>GPGSEFMGAWLRAIGLERYEEGLVHNGWDDLEFLSDITEEDLEEAGVQDPAHKRLLLDTLQLSKSSGENLYFQSSGSSGGSSGSEGVPFRTVSEWLESIKMQQYTEHFMVAGYTAIEKVVQMSNEDIKRIGVRLPGHQKRIAYSLLGLKDQVNTVGIPI[2x]

The Eph (erythropoietin-producing hepatocyte) transmembrane receptor tyrosine kinase superfamily, with its first member identified30 years ago, contains 14 members in mammals and is the largest among all receptor tyrosine kinase families. However, the cytoplasmic portion of all 14 Eph receptors are highly similar, each containing a membrane-juxtaposing kinase domain, a protein-binding SAM domain immediately followed by a short carboxyl tail PDZ domain-binding motif (PBM). In this study, we performed systematic biochemical and structural studies of the bindings of three SAM domains, two from previously identified Eph-binding proteins (SHIP2 and Odin) and one from a new Eph-binding protein discovered in this study (SAMD5), to the SAM domains from every Eph receptor. Our study reveals that the Eph SAM domains have exquisitely specific target SAM domain-binding properties, although their overall SAM-SAM heterodimer formation modes are very similar.

ITC (Isothermal Titration Calorimetry) experiment revealed that EphA2 SAM bound to SHIP2 SAM with a dissociation constant (Kd) of ~2.22 μM at a 1:1 stoichiometry. To elucidate the molecular mechanism governing the specificity of the bindings of SHIP2 SAM and Odin SAM1 to Eph receptors, we determined the crystal structure of the SHIP2 SAM-EphA2 SAM complex and the Odin SAM1-EphA6 SAM complex at the 1.5 Å and 1.3 Å resolutions, respectively. The two complex structures adopt an essentially identical End-Helix/Mid-Loop binding mode, in which positively charged residues from the N-terminal end of α5 (End-Helix) of EphA2/EphA6 bind to negatively charged residues from the loop connecting α2-α4 (Mid-Loop) from SHIP2/Odin, forming the well-known tail-to-head SAM domain heterodimer. A noticeable feature in both complexes is that the backbone methylene of a Gly residue at the beginning of α5 from Eph SAM (Gly954A2/Gly1104A6) is in close contact with an aromatic residue from SHIP2/Odin SAM (Trp1221SHIP2/Phe738Odin). Taking the EphA2/SHIP2 complex as the example, a special cation-π interaction between the Arg958A2 and Phe1226SHIP2 was uncovered by the high-resolution crystal structure. The guanidinium group of Arg958A2 forms hydrogen bond network with Asp1222SHIP2 and His955A2 on one side and with the backbone carbonyl oxygen of Ile917A2. As such the guanidinium plane of Arg958A2 (and its delocalized π-system) is in the same plane with the π-system of the planer peptide bond between Ile917A2 and Lys918A2, forming energetically favorable π-π stacking with the benzene ring of Phe1226SHIP2. Whereas the rest of Eph SAMs contain a Lys in this position except EphA10, which is an Ala. Based on the structures shown in Figure 2F, replacing Arg958A2 with Lys would eliminate the planar π-system formed by Arg958A2 and the Ile917A2-Lys918A2 peptide bond and thus seriously weaken the binding, even though the positive charge at the site is retained.>MDIGINSDPNSMKLKRLMAALTFVAAGVGAASAVAAIDPALPEYQKASGVSGNLSSVGSDTLANLMTMWAEEYKRLYPNVNIQIQAAGSSTAPPALTEGTANLGPMSRKMKDVELQAFEQKYGYKPTAVPVAVDALAIFVHKDNPIKGLTMQQVDAIFSATRLCGSKQDVKTWGDLGLTGDWAKKPVQLFGRNSVSGTYGYFKEEALCKGDFRPNVNEQPGSASVVQSVSQSLNGIGYSGIGYKTASVKTVALAKKEGAAFVEDN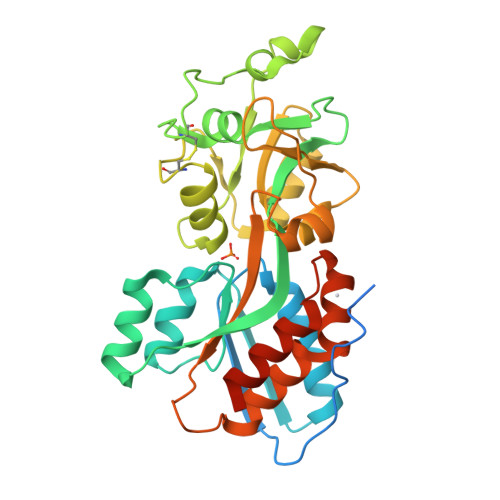EQNALNGTYPLSRFLYVYVNKAPNKPLDPLEAQFLKLVLSKTGQQVVVKDGYIPLPAKVAEKAIKELGLKLAAALEHHHHHH[4x]>[8x]MRRTVRYILATSNPMGDLEALEKFVKLAPDTGADAIALIGNLMPKAAKSRDYAAFFRILSEAHLPTAYVPGPQDAPIWEYLREAANVELVHPEMRNVHETFTFWRGPYLV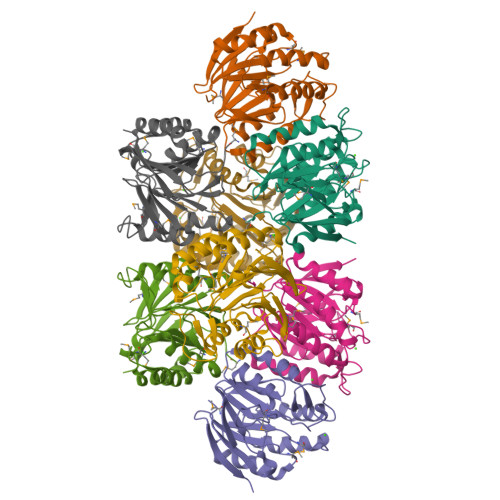AGVGGEIADEGEPEEHEALRYPAWVAEYRLKALWELKDYPKIFLFHTMPYHKGLNEQGSHEVAHLIKTHNPLLVLVAGKGQKHEMLGASWVVVPGDLSEGEYSLLDLRARKLETGNVR4-(4-methyl-1,3-thiazole-5-carbonyl)piperazin-2-one | C9 H11 N3 O2 S | 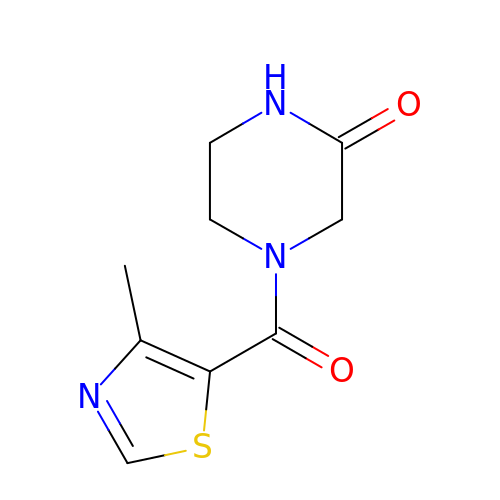CAIRNMNSCHTAFY-UHFFFAOYSA-N> ANLDIAVYWGQNFDERSLEATCDTGNYAYVIIGFLNTFGGGQTPALDISGHSPSGLEPQIKHCQSKNVKVLLSIGGPKGPYSLDSRSDANDLAVYLFNNFLLPPGHSENRPFGNAVLDGIDFHIEHGGPSQYQLLANILSSFRLAGTEFALTAAPQCVYPDPNLGTVINSATFDAIWVQFYNNPQCSYSSGNAEALMNAWREWSMKARTKKVFLGFPAHPDAAGSGYMPPE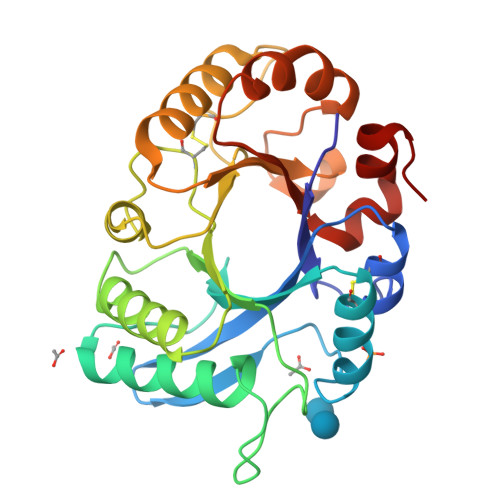KVKFHVFPAAKKSYKFGGIMLWDSYWDTVSNFSSKILGEGW> GPAKQYDSVECPFCDEVSKYEKLAKIGQGTFGEVFKARHRKTGQKVALKKVLMENEKEGFPITALREIKILQLLKHENVVNLIEICRTKASPYNRCKASIYLVFDFCEHDLAGLLSNV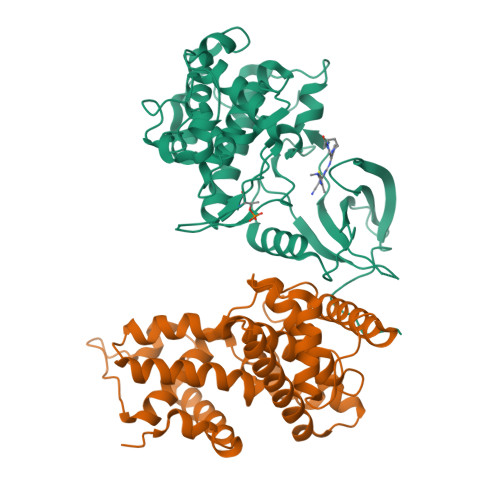LVKFTLSEIKRVMQMLLNGLYYIHRNKILHRDMKAANVLITRDGVLKLADFGLARAFSLAKNSQPNRYTNRVVTLWYRPPELLLGERDYGPPIDLWGAGCIMAEMWTRSPIMQGNTEQHQLALISQLCGSITPEVWPNVDNYELYEKLELVKGQKRKVKDRLKAYVRDPYALDLIDKLLVLDPAQRIDSDDALNHDFFWSDPMPSDLKGMLST;> GPEGERKNNNKRWYFTREQLENSPSRRFGVDPDKELSYRQQAANLLQDMGQRLNVSQLTINTAIVYMHRFYMIQSFTRFPGNSVAPAALFLAAKVEGQPKKLEHVIKVAHTCLHPQESLPDTRSEAYLQQVQDLVILESIILQTLGFELTIDHPHTHVVKCTQLVRASKDLAQTSYFMATNSLHLTTFSLQYTPPVVACVCIHLACKWSNWEIPVSTDGKHWWEYVDATVTLELLDELTHELLQILEKTPNRLKRIWNWR>[6x]MLANENSLLTMFRELGSGKLPLQIEQFERGKTIFFPGDPAERVY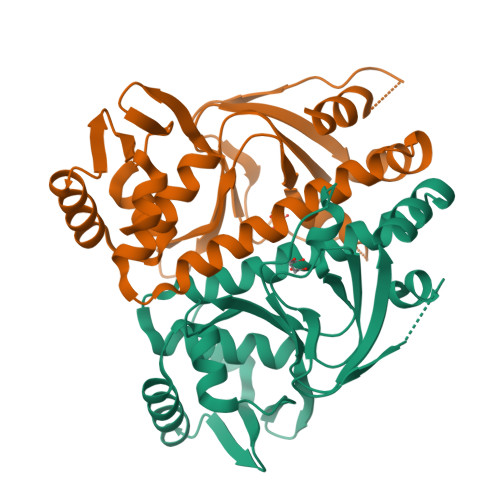LLVKGAVKLSRVYESGEEITVALLRENSVFGVLSLLTGQRSDRFYHAVAFTPVQLFSVPIEFMQKALIERPELANVMLQGLSSRILQTEMMIETLAHRDMGSRLVSFLLILCRDFGIPSPDGITIDLKLSHQAIAEAIGSTRVTVTRLLGDLRESKLIAIHKKRITVFNPVALSQQFS> MSVPTVLQKILARKAEEVAERRARVNLAEVERLARSAD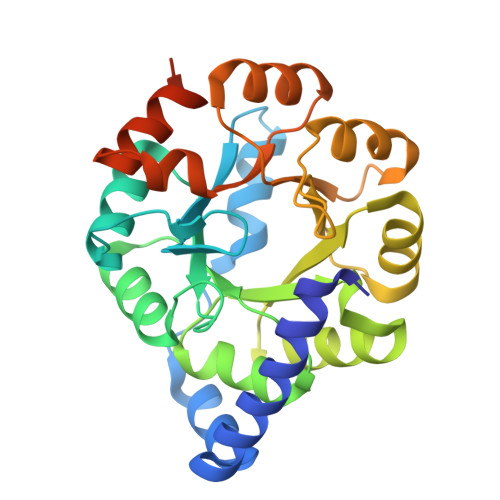APRGFANALLERAKRKEPAVIAEIKKASPSKGVLREHFVPAEIARSYEAGGAACLSVLTDVDFFQGADAYLKEARAACALPVIRKDFMIDPYQIVEARAIGADCILLIVSALDDVLMAELAATAKSVGLDVLVEVHDGTELERALKTLDTPLVGINNRNLHTFEVSLETTLDLLPEIPRDRLVVTESGILNRADVELMEVSEVYAFLVGEAFMRADDPGLELKRLFFQERGAVVLGADPDTSGHHHHHH> PAKKPYNKIVSHLLVAEPEKIYAMPDPTVPDSDIKALTTLCDLADRELVV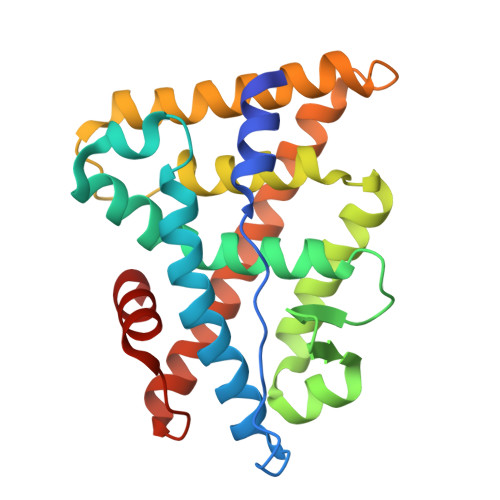IIGWAKHIPGFSTLSLADQMSLLQSAWMEILILGVVYRSLSFEDELVYADDYIMDEDQSKLAGLLDLNNAILQLVKKYKSMKLEKEEFVTLKAIALANSDSMHIEDVEAVQKLQDVLHEALQDYEAGQHMEDPRRAGKMLMTLPLLRQTSTKAVQHFYNIKLEGKVPMHKLFLEMLEAKV>[4x]MEVMNKENIIADAPSDVVKTVQQQVHLNQDEYKY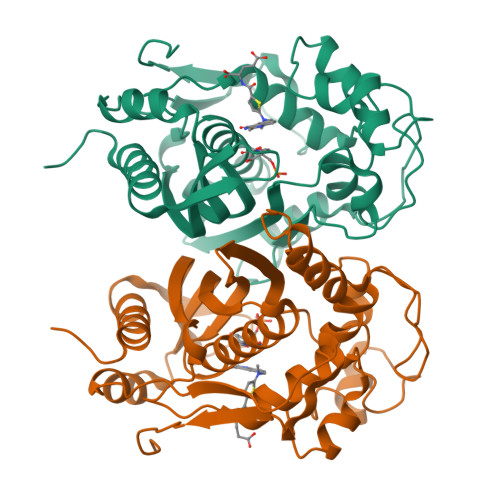LKQVEQILREGTRRDDRTGTGTISIFGMQSKYCLRNGTIPLLTTKRVYWKGVLEELLWFISGSTDGKLLMEKNVKIWEKNGDRAFLDNLGFTSREEGDLGPVYGFQWRHFGAKYVDCHTDYSGQGVDQLAEVIRQIKEQPDSRRIIMSAWNPSDLGQMVLPPCHTMCQFYVDNGELSCQLYQRSGDMGLGVPFNLASYGLLTHMIAKVCGLKPGTLVHTLGDAHVYSNHVDALKIQLDREPYAFPKIRFTRDVASIDDFTSDMIALDDYKCHPKIPMDMAV>[2x]GPLGSPEFPGSDRNSVDYAQIASGIDTRTTVMIKNIPNKFTQQMLRDYIDVTNKGTYDFLYLRIDFVNKCNVGYAFINFIEPQSIITFGKARVGTQWNVFHSEKICDISYANIQGKDRLIEKFRNSCVMDENPAYRPKIFVSHGPNRGMEEPFPAPNNARRKLRSIASAQQIGLFPPTASKC

Upon meiosis onset, Mmi1 is lured by a ribonucleoprotein (RNP) complex, composed of the nucleocytoplasmic shuttling RNA-binding protein Mei2 and the DSR-containing lncRNA meiRNA, that accumulates in a single nuclear body overlapping the meiRNA-encoding sme2 + gene. Both Mei2 and meiRNA are essential for the assembly of this structure and the completion of sexual differentiation. Interestingly, Mei2 mutants lacking the RRM3 domain (residues 592 to 750, hereafter called RRM3Mei2) failed to accumulate meiotic mRNAs, suggesting that Mei2 RNA-binding activity is required to inhibit Mmi1 function. In this study, we show that the RNA-binding activities of Mmi1 and Mei2 are crucial for their mutual control during mitosis and further identify a lncRNA, termed mamRNA, as a major regulatory and bridging partner for both proteins in the nucleus.

To gain insights into RNA recognition by RRM3Mei2, we solved its crystal structure, which revealed a unique organization as the classical RRM fold is extended by the N-terminal helix α0 and by one helix and two strands at the C-terminal extremity. Using isothermal titration calorimetry (ITC) and size exclusion chromatography coupled to multi-angle laser light scattering (SEC-MALLS), we found that RRM3Mei2 tightly interacts with a poly-U15 in a 1:1 stoichiometry.> MEGERKNNNKRWYFTREQLENSPSRRFGVDPDKELSYRQQAANLLQDMGQRLNVSQLTINTAIVYMHRFYMIQSFTQFPGNSVAPAALFLAAKVEEQPKKLEHVIKVAHTCLHPQESLPDTRSEAYLQQV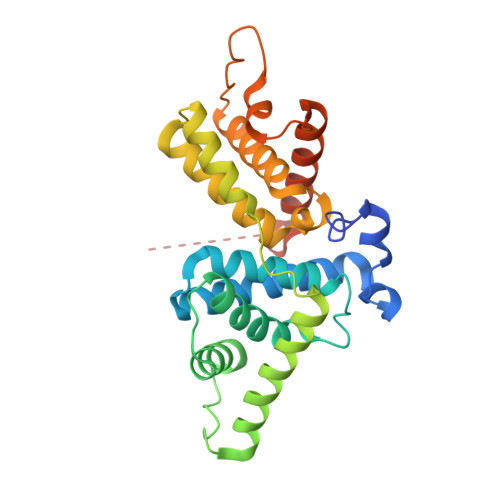QDLVILESIILQTLGFELTIDHPHTHVVKCTQLVRASKDLAQTSYFMATNSLHLTTFSLQYTPPVVACVCIHLACKWSNWEIPVSTDGKHWWEYVDATVTLELLDELTHEFLQILEKTPNRLKRIWNWRACEAAKK Our work focuses on the biopolymer poly-β(1,6)-N-acetyl-D-glucosamine (PNAG), which is produced by numerous pathogenic organisms. The final protein is PgaB, a two-domain periplasmic protein with an N-terminal family four carbohydrate esterase (CE4) domain that displays metal-dependent deacetylation activity on PNAG oligomers. Deacetylation of PNAG by the N-terminal domain of PgaB is a critical step in polymer maturation and is required for the formation of robust biofilms. Herein, we show that the C-terminal domain of PgaB is a glycoside hydrolase active on partially deacetylated PNAG, and that the enzyme disrupts PNAG-dependent biofilms and potentiates killing by antibiotics.

Bb-GH crystallized in the monoclinic space-group P21. Diffraction data were collected to 1.76 Å resolution and the structure was determined by molecular replacement. Examination of the crystal packing in the asymmetric unit revealed two Bb-GH molecules packed in a head to head fashion. We do not believe this assembly is biologically relevant as size exclusion chromatography shows that Bb-GH elutes as a monomer in solution. Bb-GH adopts a (β/α)8 barrel fold observed in GH13 family members, and also common to a wide range of other glycoside hydrolases families. Along the top face of the (β/α)8 barrel is an extended electronegative groove that is approximately 43 Å long and 11 Å wide. There is also a defined pocket at the center of the groove. This central pocket and most of the electrostatic groove contain residues that are highly conserved among orthologues. Taken together, the mutagenesis data suggests that residues D326, D328, D364, and E585 play a role in substrate binding as the asparagine or glutamine mutants displayed detectable activity, while D474 is the most probable residue to be involved in catalysis as it is the only residue whose activity is ablated in both the asparagine and alanine variants. Considering that neither PgaBBb nor PgaBEc have sequence or structural similarity to the active site to DspB or other closely related GH family members, we propose that the C-terminal domain of PgaB defines a new GH family, GH153.

>GSHMPIERIVQVDLDYIYDPDPEQQNRNLGQLIDRMKDLAPSAVYLQAFADPKGDGDITEVYFPNRHLPMRADLFNRVAWQLKTRAGVMVYAWLPVLTFSVPPGNPAYGKVVQSTTRKPGERGLGSPTRLSPFHPDAHRVISEIYEDLAKAAHFDGLLFHDDAVLDDTEDSSPEALATYQGWGLPPDIAAIRADPKLAQQWSKGKIRYLIDFTMHLRHIVSGYQNDRDMVVARNLYAQPVLDPVSEAWYGQSLPEFLKSYDFVALMAMPNMEGAARPEQWMRQLVAAVARQKGLDRTIFELQARDWRVGKPIDTEILRRQMVQLRSLGAINYGYYPDDFIANHPDAEALRDVMSLKS[2x]>[4x]MTS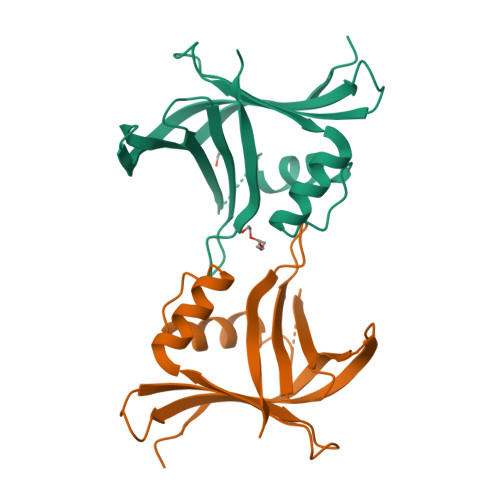KIALFDQTLIASLLQPLSLNQPDFKAYKTKVKLKISEQRNETSGEKELKFEISRSDDFEFLFSETLNNEKYQILARDHDLTVDFDAFPKVIIQHLLCKNIVKNLEEDGEVDARKKAGYHEIADPGKPTEINIILDAEKNFCSFELFSKTPWSKGKIFSIKLHAVR> ELTGFEPYDYQLRAWEKIREIM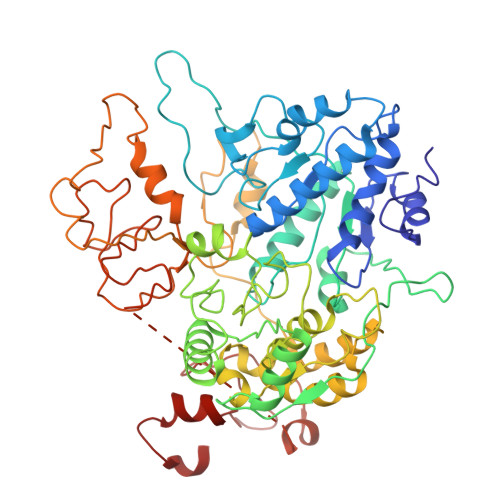NNGGKVIIEVPTAGGKTETAVMPFFAGIYNNNWPVARLVYVLPTRSLVEKQAERLRNLVYKLLQLKGKSKEEAEKLARELVVVEYGLEKTHAFLGWVVVTTWDAFLYGLAAHRTVGNRFTFPAGAIAQSLVIFDEVQMYQDESMYMPRLLSLVVGILEEANVPLVIMSATIPSKLREMIAGDTEVITVDKNDKNKPSKGNVKVRLVEGDITDVLNDIKKILKNGKKVLVVRNTVRKAVETYQVLKKKLNDTLANPSDALLIHSRFTIGDRREKERALDSARLIVATQVVEAGLDLPNVGLVVTDIAPLDALIQRIGRCARRPGEEGEGIILIPAAAAAAAAAAAAAAAAAAAAAAAAAAAAVVTSTNEYDRVVEIHYGEGKKNFVYVGDIDTARRVLEKKRSKKLPKDLYIIPYSVSPYPDPLVLLTTYDELSKIGEYLADTTKARKALDRVYKFHYENNIVPKEFASYIYFKELKLFSAPPEYEKAAAAAAAAAAAAAAAAAAAAAAAAAAAAAAAAAAAIDAKYYNSELAAAAAAAAAAAAAAAAAAA> MIKVEIKPSQAQFTTRSGVSRQGKPYSLNEQLC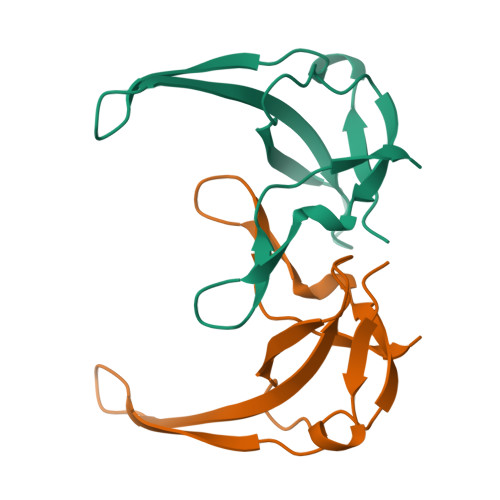YADLGNEYPVLVKLTLDEGQPAYAPGLYTVHLSSFKVGQFGSLMIDRLRLVPAK> APAVADKADNAFMMICTALVLFMTIPGIALFYGGLIRGKNVLSMLTQVTVTFALVCILWVVYGYSLAFGEGNNFFGNINWLMLKNIELTAVMGSIYQYIHVAFQGSAACITVGLIVGALAERIRFSAVLIFVVVWLTLSYIPIAHMVWGGGLLASHGALDFAGGTVVHINAAIA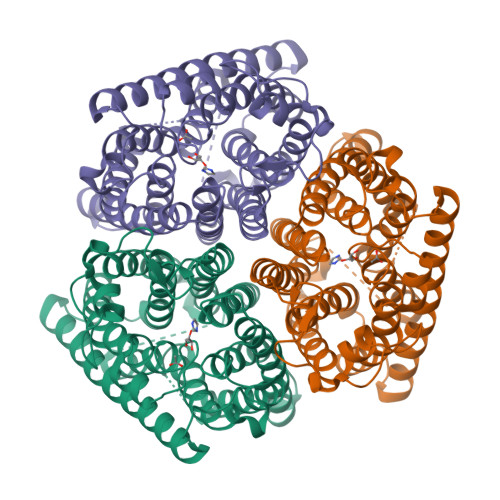GLVGAYLIGKRVGFGKEAFKPHNLPMVFTGTAILYIGWFGANAGSAGTANEIAALAFVNTVVATAAAILGWIFGEWALRGKPSLLGACSGAIAGLVGVTPACGYIGVGGALIIGVVAGLAGLWGVTMLKRLLRVDDPCDVFGVHGVCGIVGCIMTGIFAASSLGGVGFAEGVTMGHQLLVQLESIAITIVWSGVVAFIGYKLADLTVGLRVPEEQEREGLDVNSHGENAYNADQAQQPAQADLEHHHHHH> RTP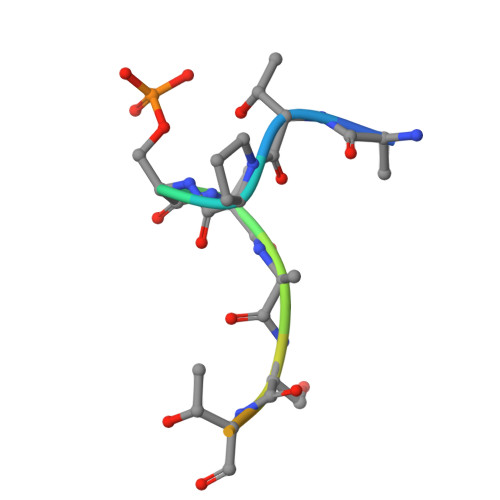SSASTVSVGY> MEQKLISEEDLGGGEQKLISEEDLGGGEQKLISEEDLGGGMDKDCEMKRTTLDSPLGKLELSGCEQGLHRIIFLGKGTSAADAVEVPAPAAVLGGPEPLIQATAWLNAYFHQPEAIEEFPVPALHHPVFQQESFTRQVLWKLLKVVKFGEVISESHLAALVGNPAATAAVNTALDGNPVPILIPCHRVVQGDSDVGPYLGGLAVKEWLLAHEGHRLGKPGLGGGSGMATRGANVIWFRHGLRLHDNPALLAALADKDQGIALIPVFIFDGESAGTKNVGYNRMRFLLDSLQDIDDQLQAATDGRGRLLVFEGEPAYIFRRLHEQVRLHRICIEQDCEPIWNERDESIRSLCRELNIDFVEKVSHTLWDPQLVIETNGGIPPLTYQMFLHTVQIIGLPPRPTADARLEDATFVELDPEFCRSLKLFEQLPTPEHFNVYGDNMGFLAKINWRGGETQALLLLDERLKVEQHAFERGFYLPNQALPNIHDSPKSMSAHLRFGCLSVRRFYWSVHDLFKNVQLRACVRGVQMTGGAHITGQLIWREYFYTMSVNNPNYDRMEGNDICLSIPWAKPNENLLQSWRLGQTGFPLIDGAMRQLLAEGWLHHTLRNTVATFLTRGGLWQSWEHGLQHFLKYLLDADWSVCAGNWMWVSSSAFERLLDSSLVTCPVALAKRLDPDGTYIKQYVPELMNVPKEFVHEPWRMSAEQQEQYECLIGVHYPERIIDLSMAVKRNMLAMKSLRNSLITPP;> MDWLLATPQLYSAFSSLGCLEGDTYVVNPNALAILEEINYKLTYEDQTLRTFRRAIGFGQNVRSDLIPLLENAKDDAVLESVIRILVNLTVPVECLFSVDVMYRTDVGRHTIFELNKLLYTSKEAFTEARSTKSVVEYMKHILESDPKLSPHKCDQINNCLLLLRNILHIPETHAHCVMPMMQSMPHGISMQNTILWNLFIQSIDKLLLYLMTCPQRAFWGVTMVQLIALIYKDQHVSTLQKLLSLWFEASLSESSEDNESNTSPPKQGSGDSSPMLTSDPTSDSSDNGSNGRGMGGGMREGTAATLQEVSRKGQEYQNAMARVPADKPDGSEEASDMTGNDSEQPGSPEQSQPAGESMDDGDYEDQRHRQLNEHGEEDEDEDEVEEEEYLQLGPASEPLNLTQQPADKVNNTTNPTSSAPQGCLGNEPFKPPPPLPVRASTSAHAQMQKFNESSYASHVSAVKLGQKSPHAGQLQLTKGKCCPQKRECPSSQSELSDCGYGTQVENQESISTSSNDDDGPQGKPQHQKPPCNTKPRNKPRTIMSPMDKKELRRKKLVKRSKSSLINMKGLVQHTPTDDDISNLLKEFTVDFLLKGYSYLVEELHMQLLSNAKVPIDTSHFFWLVTYFLKFAAQLELDMEHIDTILTYDVLSYLTYEGVSLCEQLELNARQEGSDLKPYLRRMHLVVTAIREFLQAIDTYNKVTHLNEDDKAHLRQLQLQISEMSDLRCLFVLLLRRFNPSIHSKQYLQDLVVTNHILLLILDSSAKLGGCQTIRLSEHITQFATLEVMHYYGILLEDFNNNGEFVNDCIFTMMHHIGGDLGQIGVLFQPIILKTYSRIWEADYELCDDWSDLIEYVIHKFMNTPPKSPLTIPTTSLTEMTKEHNQEHTVCSWSQEEMDTLYWYYVQSKKNNDIVGKIVKLFSNNGNKLKTRISIIQQLLQQDIITLLEYDDLMKFEDAEYQRTLLTTPTSATTESGIEIKECAYGKPSDDVQILLDLIIKENKAQHLLWLQRILIECCFVKLTLRSGLKVPEGDHIMEPVAYHCICKQKSIPVVQWNNEQSTTMLYQPFVLLLHKLGIQLPADAGSIFARIPDYWTPETMYGLAKKLGPLDKLNLKFDASELEDATASSPSRYHHTGPRNSLSSVSSLDVDLGDTEELALIPEVDAAVEKAHAMASTPSPSEIFAVPKTKHCNSIIRYTPDPTPPVPNWLQLVMRSKCNHRTGPSGDPSDCIGSSSTTVDDEGFGKSISAATSQAASTSMSTVNPTTTLSLNMLNTFMGSHNENSSSSGCGGTVSSLSMVALMSTGAAGGGGNTSGLEMDVDASMKSSFERLEVNGSHFSRANNLDQEYSAMVASVYEKEKELNSDNVSLASDLTRMYVSDEDDRLERTEIRVPHYHLEGGSGMDKDCEMKRTTLDSPLGKLELSGCEQGLHRIIFLGKGTSAADAVEVPAPAAVLGGPEPLMQATAWLNAY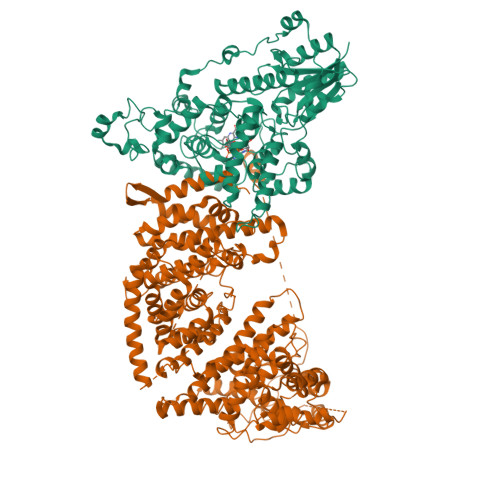FHQPEAIEEFPVPALHHPVFQQESFTRQVLWKLLKVVKFGEVISYSHLAALAGNPAATAAVKTALSGNPVPILIPCHRVVQGDLDVGGYEGGLAVKEWLLAHEGHRLGKPGLGGGGYPYDVPDYARTGGGSGSRLEEELRRRLTE>[3x]ASNFTQFVLVDNGGTGDVTVAPSNFANGVAEWISSNSRSQAYKVTCSVRQSSA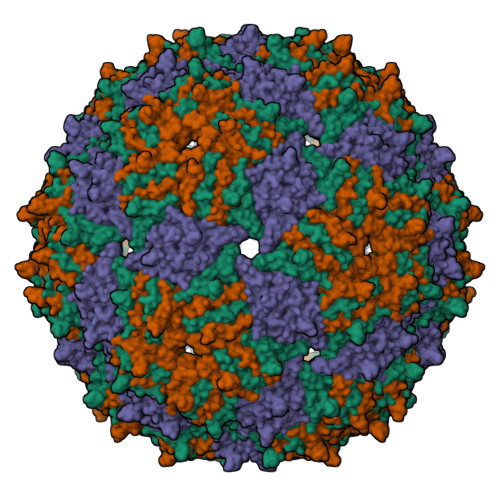QNRKYTIKVEVPKVATQTVGGVELPVAAWRSYLAMELTIPIFATNSDCELIVKAMQGLLKDGNPIPSAIAANSGIY>[8x]MSTHSSTVQNDLAALIHPNTNLAQHREVGPLVIARGDGVRVFDEQGNAYIEAMSGLWSAALGFSEQRLVDAAVEQFKQLPYYHSFSHKTNAPAAALAAKLAALAPGDLNHVFFTNSGSEANDSVVKMVWYVNNALGRPAKKKFISRQQAYHGATVAAASLTGIPSMHRDFDLPAIPVHHLTCPNFYRFARPGESQEAFTVRLANELERYILAEGPETIAAFIGEPVIAAGGVIPPPTGYWAAIQAVCKRYDILVVIDEIITGFGRLGTMFGSQLYGIQPDIMVLSKQLTSSYQPLAAVVVSDAMNDVLVSQSQRLGAFAHGFTCTGHPVATAVALENIRIIEERDLVGHVQHLAPVFQRHLRAFEDHPLVGNVRGVGLMGGIELVADKATRQPFAQPGTLGGYVFKQAHKHGLIIRAIYDTIAFCPPLITTQDDIEAIFSAFERTLADATDWARSQHLL

Omega transaminases (ω-TAs) can mediate the chiral amination of several unnatural substrates without the requirement of an α-COOH group and are highly relevant in the production of several pharmaceutical intermediates of commercial interest. In this work, we successfully overexpressed and characterized the two recombinant transaminases TA_2799 and TA_5182 from P. putida KT2440 and solved their crystal structures. The overall structural fold of the TA_5182 and TA_2799 enzymes is similar to that observed for other class III fold type I TAs with two α/β domains. There are two highly flexible loops present in the structures of TA_2799 and TA_5182 that mediate the entry and exit of the cofactor and the substrate/byproduct into the active site of the enzyme, leading to significant conformational changes in the enzyme structure.

The crystal structure of L322F mutant of TA_2799 was solved at a resolution of 2.5 Å. The TA_2799_L322F mutant was crystallized in its apo form, with a sulfate ion bound in the phosphate-binding pocket of the enzyme. We expected PLP electron density in the crystal structure of the TA_2799_L322F mutant; however, only sulfate ion density could be seen. PLP may have been present at the active site, but not covalently bound as an internal aldimine, and thus, the sulfate ions from the crystallization mother liquor could compete and displace the PLP molecule out of the active site pocket. In the crystal structure of the TA_2799_L322F mutant enzyme, the ND1 of the N121 residue maintains hydrogen bonds with both OE1 and OE2 of E123, which provides further stability to the anion-pi stacking interaction between E123 and F322 in the same monomer. Apart from that, the OE1 of E123 forms a hydrogen bond with OG of S120, forming an extensive intersubunit network that stabilizes the dimer. The effect of the L322F mutation is observed in the thermal stability assay, as the mutant enzyme has an increased ∼6 °C melting temperature (Tmapp) over the wild-type TA_2799. The mutant enzyme’s affinity towards the cofactor PLP is clearly enhanced as observed by the yellow coloration of the enzyme solution post-purification and the characteristic peak for PLP at 420 nm seen in the absorbance spectra of the purified enzyme, similar to the report of Kwon et al.. The mutant enzyme efficiently converts (R)-PAC to (1R, 2S)-NE even without external cofactor addition to the reaction mixture. The TA_2799_L322F mutant showed the best increase in stability; it retained ∼70% of its activity even after 96h of storage.> SNPTTFSVEAIAAYTPVALIRLLNASGPLQPGHRVDIADARSIYTVGAAASAARARANHNANTIRRTAMFAETDPMTWLRP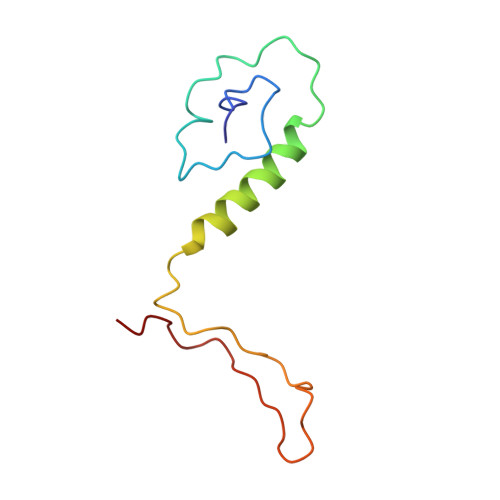TVGLRRTFNPRII>RGLASKKTTTVGVIIPDISNIFYAELARGIEDIATMYKYNIILSNSDQNQDKELHLLNNMLGKQVDGIIFMSGNVTEEHVEELKKSPVPVVLAASIESTNQIPSVTIDYEQAAFDAVQSLIDSGHKNIAFVSGTLEEPINHAKKVKGYKRALTESGLPVRDSYIVEGDYTYDSGIEAVEKLLEEDEKPTAIFVGTDEMALGVIHGAQDRGLNVPNDLEIIGFDNTRLSTMVRP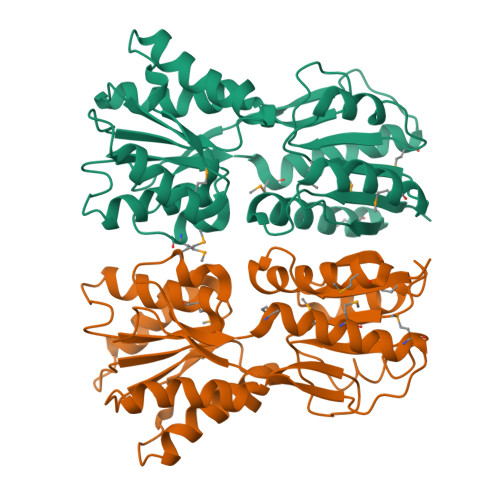QLTSVVQPMYDIGAVAMRLLTKYMNKETVDSSIVQLPHRIEFRQSTK[2x]Uropathogenic Escherichia coli strains use filamentous type 1 pili to adhere to and invade uroepithelial cells. The pilus consists of a flexible tip fibrillum, formed by the adhesin FimH and the subunits FimG and FimF. The pilus rod is a helical assembly of up to 3000 copies of the main subunit FimA, terminated by a single copy of the subunit FimI that anchors the rod to the assembly platform FimD in the outer membrane. The assembly platform FimD in the outer membrane of uropathogenic E. coli is the catalyst of type 1 pilus assembly.

To explore the structural implications of FimI-mediated termination of pilus assembly, we performed a FimD-catalyzed assembly reaction of pilus rods in vitro similar to the one for the FimDHGFAnC complex, except that excess FimICHis was also added at the end of the reaction. Given the low FimI concentrations in the periplasm (FimA:FimI ratio ≥100:1), we focused our analysis on physiological pilus complexes with a single terminal FimI subunit capped by FimCHis. A 3D reconstruction of the FimDHGFAnICHis complex at 6.4 Å resolution was generated (Map XIV). However, multi-body refinement with blush regularization in RELION-5.033,34 improved the resolution to 4.0 Å for the pilus rod (map XV) and 4.3 Å for the FimI-bound assembly platform (map XVI). The resulting composite model shows that the FimI-terminated pilus rod sits on top of the assembly platform at an angle of about 48°, similar to that observed for the FimDHGFAnC complex. In addition, the comparison of the complexes with and without FimI showed that the subunit in the usher pore and the FimC-complemented subunit on the periplasmic side occupy nearly the same positions when the two structures are aligned based on the transmembrane and plug domains of the usher (RMSD = 0.56 Å). The overall conformation of the usher also remains unchanged between the FimA and the FimI-bound states. In contrast to the major conformational changes observed in early steps of pilus assembly after plug domain displacement, no major conformational changes were detected in the transmembrane domain of FimD upon incorporation of FimI. We then aligned the FimDHGFAnICHis complex (model XVI) to the previously crystallized FimAICHis complex (PDB-ID 6SWH20) via FimC to assess structural differences. The angle between FimA and FimI differed: in the isolated FimAICHis complex, which is not restrained by FimD, FimI adopts a slightly different angle that would cause a clash with the transmembrane domain of FimD.

> MAATTVNGGTVHFKGEVVNAACAVDAGSVDQTVQLGQVRTASLAQEGATSSAVGFNIQLNDCDTNVASKAAVAFLGTAIDAGHTNVLALQSSAAGSATNVGVQILDRTGAALTLDGATFSSETTLNNGTNTIPFQARYFATGAATPGAANADATFKVQYQ;> MGVALGATRVIYPAGQKQEQLAVTNNDENSTYLIQSWVENADGVKDGRFIVTPPLFAMKGKKENTLRILDATNNQLPQDRESLFWMNVKAIPSMDKSKLTENTLQLAIISRIKLYYRPAKLALPPDQAAEKLRFRRSANSLTLINPTPYYLTVTELNAGTRVLENALVPPMGESTVKLPSDAGSNITYRTINDYGALTPKMTGVMEHHHHHH;> DLYFNPRFLADDPQAVADLSRFENGQELPPGTYRVDIYLNNGYMATRDVTFNTGDSEQGIVPCLTRAQLASMGLNTASVAGMNLLADDACVPLTTMVQDATAHLDVGQQRLNLTIPQAFMSNRARGYIPPELWDPGINAGLLNYNFSGNSVQNRIGGNSHYAYLNLQSGLNIGAWRLRDNTTWSYNSSDRSSGSKNKWQHINTWLERDIIPLRSRLTLGDGYTQGDIFDGINFRGAQLASDDNMLPDSQRGFAPVIHGIARGTAQVTIKQNGYDIYNSTVPPGPFTINDIYAAGNSGDLQVTIKEADGSTQIFTVPYSSVPLLQREGHTRYSITAGEYRSGNAQQEKPRFFQSTLLHGLPAGWTIYGGTQLADRYRAFNFGIGKNMGALGALSVDMTQANSTLPDDSQHDGQSVRFLYNKSLNESGTNIQLVGYRYSTSGYFNFADTTYSRMNGYNIETQDGVIQVKPKFTDYYNLAYNKRGKLQLTVTQQLGRTSTLYLSGSHQTYWGTSNVDEQFQAGLNTAFEDINWTLSYSLTKNAWQKGRDQMLALNVNIPFSHWLRSDSKSQWRHASASYSMSHDLNGRMTNLAGVYGTLLEDNNLSYSVQTGYAGGGDGNSGSTGYATLNYRGGYGNANIGYSHSDDIKQLYYGVSGGVLAHANGVTLGQPLNDTVVLVKAPGAKDAKVENQTGVRTDWRGYAVLPYATEYRENRVALDTNTLADNVDLDNAVANVVPTRGAIVRAEFKARVGIKLLMTLTHNNKPLPFGAMVTSESSQSSGIVADNGQVYLSGMPLAGKVQVKWGEEENAHCVANYQLPPESQQQLLTQLSAECRLVPRGSWSHPQFEK;> GNKWNTTLPGGNMQFQGVIIAETCRIEAGDKQMTVNMGQISSNRFHAVGEDSAPVPFVIHLRECSTVVSERVGVAFHGVADGKNPDVLSVGEGPGIATNIGVALFDDEGNLVPINRPPANWKRLYSGSTSLHFIAKYRATGRRVTGGIANAQAWFSLTYQ>[8x]GSFVGSIDQGTTSSRFLIFNGEGNPVASHQIEFENLYPKSGWHEQDPYELLNSVQQCIDGAMHKFASLGYSKENIRAIGITNQRETTVVWDSVTGEPLHNAIVWPDTRTSALVRELKARQSADSLLELCGLPLSTYPSSVKLLWLIQNVDAVKQAYEEGRLAFGTVDSWLIYKLNGGAQAERPIHVTDSTNASRTMFMNLRTLQYDDKLLGFFGIDRNKIKLPKIVPSSDPEAFGKVATGALAGVPIAGCLGDQSSALVGQCGFSPGQAKNTYGTGCFLLYNVGTEPVISKYGLLATVAYDFGRGRKPVYALEGSIAVAGAGITFLMNNLGFAPKPSEINALAESVLDNGGVVFVTAFSGLFAPYWIDDAKGTLFGITQHTTKGHIARATLEATCYQTRAILDAMEKDSGHKLESLAVDGGLSASDLCMQTQADISGIPVDRPRMRETTALGAAIAAGLATGVWRELDHVKESIAGGANGNGKKNAREVFYPKMDRKKAERLFRKWEQAVEMSRGWVREQEEEDGE

Here, we report the first structure of glycerol kinase from the thermophilic filamentous fungus Chaetomium thermophilum (CtGK). Glycerol kinase (EC 2.7.1.30) catalyzes the transfer of phosphate moiety from ATP to glycerol to form glycerol 3-phosphate (G3P). Overall, the CtGK polypeptide chain can be divided into two distinct domains classified by Pfam as FGGY_N (residues 65–325) and FGGY_C (residues 331–583) connected by a flexible region. A similar case is found in CtGK, which forms extended dimers via the interaction between the C-terminal domains with a prominent contribution from hydrophobic residues (Phe422, Gly436, Phe389, Leu394, Thr437, Phe439, Gly440, Ile441, Thr437, Thr445, Leu438, Ile450, Trp580).

Subsequently, by replacing the cryoprotectant solution with 20–25% glycerol, we were able to solve the enzyme-substrate complex with a clear electron density that could be attributed to the bound glycerol moiety. In total, three different crystal structures were obtained in the presence of glycerol, constituting 13 polypeptide chains. Generally, the same extent of the chain could be modeled as in the apo structures, i.e., for residues 65–583 with an approximate 9aa gap between H18 and B18. The substrate is bound in an evolutionarily conserved cleft within the N-terminal domain that opens towards the C-terminal domain. The glycerol molecule is coordinated by polar interactions with side chains of Glu149, Arg 148, Asp317, Gln318, and additionally with Arg148 main-chain amide. The carbon chain of glycerol packs against hydrophobic Trp168 and Phe342. A similar mode of binding was described previously for P. falciparum GK, where Phe271 and Tyr135 undergo shift upon substrate or cofactor binding. However, the movement of equivalent residues (Phe342 and Tyr200) was not observed in either of the presented CtGK complexes. Of note, we solved and refined five CtGK structures, and each of them belongs to a different space group, despite crystals having grown in the same buffer condition. We observed that in the absence of nucleotide, CtGK adopts open conformation, which upon nucleotide binding closes up.>MTETASVALIENLQREELSSIEEAHAYARLLELHDLTQEALAQRLGKGQSTIANKLRLLKLPQPVQEAIMEKKITERHARALIPLKQPELQVTLLTEII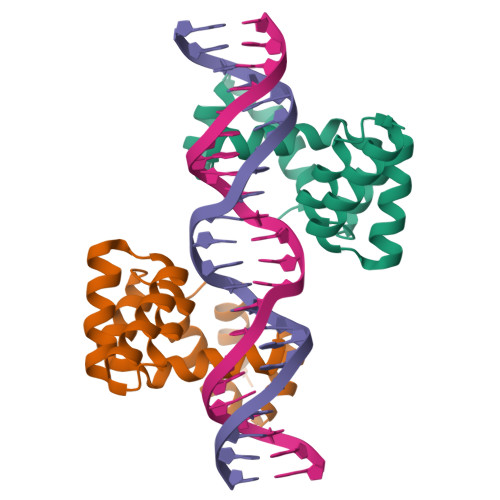EKSLNVKQTEDRVVKMLEQGQRKPKPRRKAFSRDKLAAALEHHHHHH[2x]>[2x]GMAPDQQVPATALGKSSRISLDGRRSERSVILADGSMHSLTLLHPGVYTLS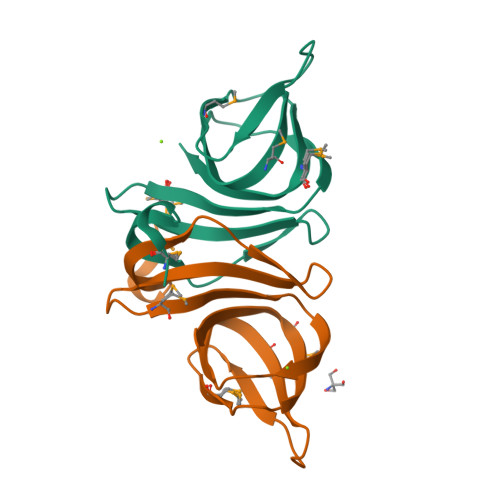SEVAETIRVLSGMAYYHAEGANDVQELHAGDSMVIPANQSYRLEVMEPLDYLLSS>[3x]MPDFLGHAENPLREEEWARLNETVIQVARRSLVGRRILDIYGPLGAGVQTVPYDEFQGVSPGAVDIVGEQETAMVFTDARKFKTIPIIYKDFLLHWRDIEAARTHNMPLDVSAAAGAAALCAQQEDELIFY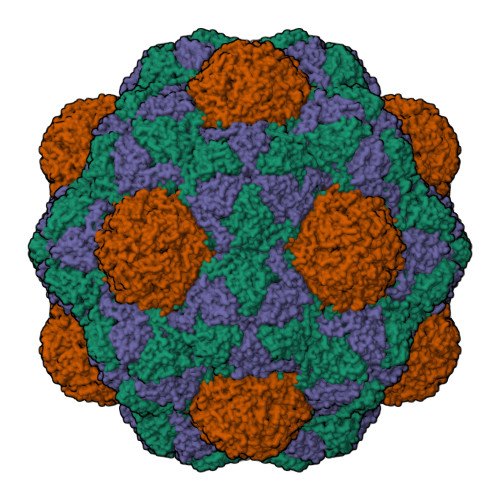GDARLGYEGLMTANGRLTVPLGDWTSPGGGFQAIVEATRKLNEQGHFGPYAVVLSPRLYSQLHRIYEKTGVLEIETIRQLASDGVYQSNRLRGESGVVVSTGRENMDLAVSMDMVAAYLGASRMNHPFRVLEALLLRIKHPDAICTLEGAGATERR;>MGPGSDKDCEMKRTTLDSPLGKLELSGCEQGLHEIIFLGKGTSAADAVEVPAPAAVLGGPEPLMQATAWLNAYFHQPEAIEEFPVPALHHPVFQQESFTRQVLWKLLKVVKFGEVISYSHLAALAGNPAATAAVKTALSGNPVPILIPCHRVVQGDLDVGGYEGGLAVKEWLLAHEGHRLGKRGGGSGGGSPEKRLTVGSLRR[3x]> MKILILGIFLFLCSTPAWAKEKHYYIGIIETTWDYASDHGEKKLISVDTEHSNIYLQNGPDRIGRLYKKALYLQYTDETFRTTIEKPVWLGFLGPIIKAETGDKVYVHLKNLASRPYTFHSHGITYYKEHEGAIYPDNTTDFQRADDKVYPGEQYTYMLLATEEQSPGEGDGNCVTRIYHSHIDAPKDIASGLIGPLIICKKDSLDKEKEKHIDREFVVMFSVVDENFSWYLEDNIKTYCSEPEKVDKDNEDFQESNRMYSVNGYTFGSLPGLSMCAEDRVKWYLFGMGNEVDVHAAFFHGQALTNKNYRIDTINLFPATLFDAYMVAQNPGEWMLSCQNLNHLKAGLQAFFQVQECNKSSSKDNIRGKHVRHYYIAAEEIIWNYAPSGIDIFTKENLTAPGSDSAVFFEQGTTRIGGSYKKLVYREYTDASFTNRKERGPEEEHLGILGPVIWAEVGDTIRVTFHNKGAYPLSIEPIGVRFNKNNEGTYYSPNYNPQSRSVPPSASHVAPTETFTYEWTVPKEVGPTNADPVCLAKMYYSAVDPTKDIFTGLIGPMKICKKGSLHANGRQKDVDKEFYLFPTVFDENESLLLEDNIRMFTTAPDQVDKEDEDFQESNKMHSMNGFMYGNQPGLTMCKGDSVVWYLFSAGNEADVHGIYFSGNTYLWRGERRDTANLFPQTSLTLHMWPDTEGTFNVECLTTDHYTGGMKQKYTVNQCRRQSEDSTFYLGERTYYIAAVEVEWDYSPQREWEKELHHLQEQNVSNAFLDKGEFYIGSKYKKVVYRQYTDSTFRVPVERKAEEEHLGILGPQLHADVGDKVKIIFKNMATRPYSIHAHGVQTESSTVTPTLPGETLTYVWKIPERSGAGTEDSACIPWAYYSTVDQVKDLYSGLIGPLIVCRRPYLKVFNPRRKLEFALLFLVFDENESWYLDDNIKTYSDHPEKVNKDD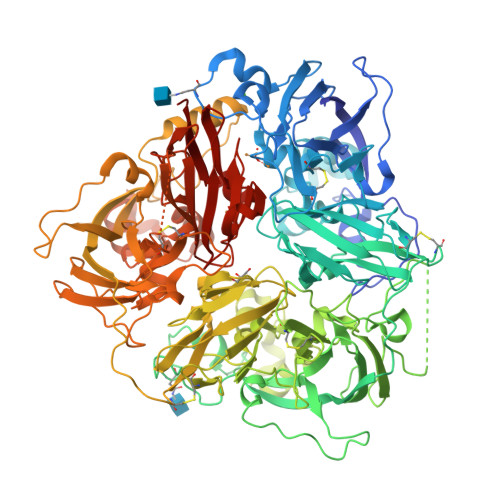EEFIESNKMHAINGRMFGNLQGLTMHVGDEVNWYLMGMGNEIDLHTVHFHGHSFQYKHRGVYSSDVFDIFPGTYQTLEMFPRTPGIWLLHCHVTDHIHAGMETTYTVLQNEDTKSG> SNATSRKKVLLKVIILGDSGV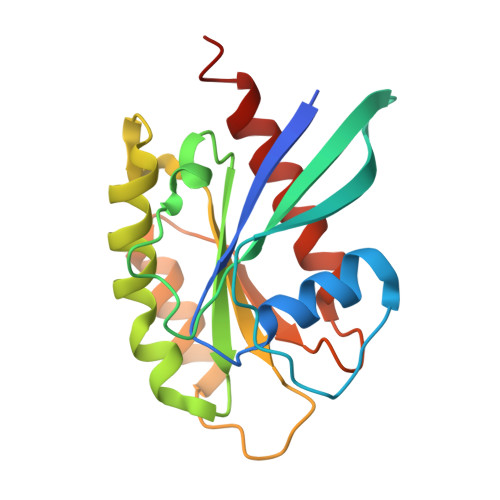GKTSLMNQYVNKKFSNQYKATIGADFLTKEVMVDDRLVTMQIWDTAGLERFQSLGVAFYRGADCCVLVFDVTAPNTFKTLDSWRDEFLIQASPRDPENFPFVVLGNKIDLENRQVATKRAQAWCYSKNNIPYFETSAKEAINVEQAFQTIARNALKQETEVEL>GPSGGGADVNKGPWAMALTPMEFARKYNLLRKDDALLDNPVPGEEMTAGIRRGDAKRVFTMQLGPYWDGFERCSPQAYALSAVFMARMNRDRDAANNILKVLDKTFVDGKPDFSVARPVMKKYQNSELVQEVVAKHAYVLTVIASLLEAAREDGVVPSSEFLWLKPVDEELWYMLNCVGRQTPYSEVAGPFAH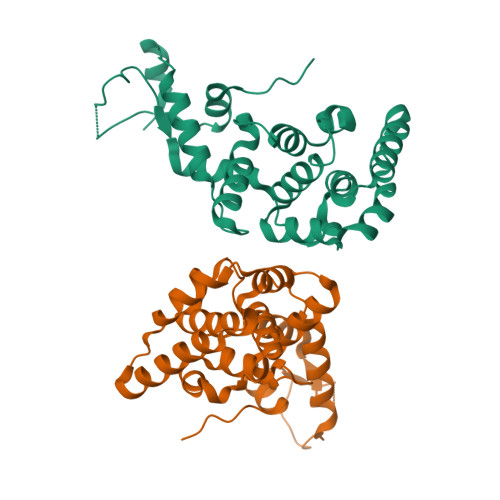WKAEKEMGRRSLVPMIDEAIRALEIAVKEVRLTPRQMEELEP[2x]>[2x]MAKSKFEYVRDFEADDTCLAHCWVVVRLDGRNFHRFAEKHNFA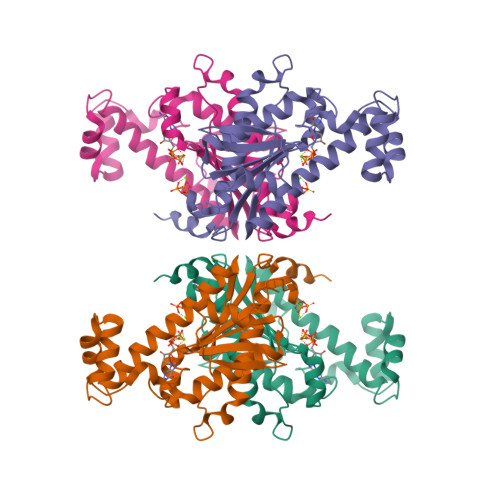KPNDSRALQLMTKCAQTVMEELEDIVIAYGQSDEYSFVFKRKTNWFKRRASKFMTHVASQFASSYVFYWRDYFEDQPLLYPPGFDGRVVVYPSNQTLKDYLSWRQADCHINNLYNTVFWALIQQSGLTPVQAQGRLQGTLAADKNEILFSEFNINYNNELPMYRKGTVLIWQKVDEVMTKEIKLPTEMEGKKMAVTRTRTKPVPLHCDIIGDAFWKEHPEILDEDS Two Agrobacterium ABC-transporters and their cognate periplasmic binding proteins (PBPs) OccJ and NocT import octopine and nopaline/octopine, respectively. Recognition and import of opines are conferred by periplasmic binding proteins (PBPs) and their associated ATP-binding cassette (ABC) transporters. The PBP OccJ is associated with the octopine transporter of octopine-type A. tumefaciens while NocT is associated with nopaline uptake in the nopaline-type A. tumefaciens. OccJ shares 47% sequence identity with NocT and belongs to cluster F within the PBP structural classification.

In contrast, we were successful in solving the structures of NocT with octopinic acid, noroctopinic acid and histopine at 2.1, 2.2 and 2.45 Å resolution, respectively. All ligands are well defined in their electron density maps. Octopinic acid and noroctopinic acid contain an ornithine moiety instead of the arginine for octopine. Local rearrangements of residues in the ligand binding site such as Glu36, Ala94, Met117 and those from the region 165–170 occur upon octopinic acid, noroctopinic acid and histopine binding compared with octopine, with Glu36 and Gln165 moving towards both shortest side chains of ornithine and histidine moieties. The ornithine moiety forms fewer polar interactions with the protein than the arginine moiety. In contrast, the pyruvate of the octopinic acid and histopine as well as the glyoxylic acid (a CH3 shorter than pyruvate) of noroctopinic acid adopt a similar position, comparable to that of the pyruvate of octopine. The same study performed with NocT showed that NocT displays similar affinity for octopine and its family members except for histopine, which is the worst ligand as for OccJ. The structural data of NocT with octopinic acid, histopine and an octopine analogue confirm a unique binding mode with a unique conformation of the ketoacid moiety, which is different from that observed in OccJ.

>[2x]MKDYKSITIATEGSYAPYNFKDAGGKLIGFDIDLGNDLCKRMNIECKFVEQAWDGIIPSLTAGRYDAIMAAMGIQPAREKVIAFSRPYLLTPMTFLTTADSPLLKTQVAIENLPLDNITPEQKAELDKFTKIFEGVKFGVQAGTSHEAFMKQMMPSVQISTYDTIDNVVMDLKAGRIDASLASVSFLKPLTDKPDNKDLKMFGPRMTGGLFGKGVGVGIRKEDADLKALFDKAIDAAIADGTVQKLSQQWFGYDASPKQHHHHHH> KVFGITGPVSTVGATAAENKLNDSLIQELKKEGSFETEQETANRVQVLKILQELAQRFVYEVSKKKNMSDGMARDAGGKIFTYGSYRLGVHGPGSDIDTLVVVPKHVTREDFFTVFDSLLRERKELDEIAPVPDAFVPIIKIKFSGISIALICARLDQPQVPLSLTLSDKNLLRNLDEKDLRALNGTRVTDEILELVPKPNVFRIALRAIKLWAQRRAVYANIFGFPGGVAWAMLVARICQLYPNACSAVILNRFFIILSEWNWPQPVILKPIEDGPLQVRVWNPKIYAQDRSHRMPVITPAYPSMCATHNITESTKKVILQEFVRGVQITNDIFSNKKSWANLFEKNDFFFRYKFYLEITAYTRGSDEQHLKWSGLVESKVRLLVMKLEVLAGIKIAHP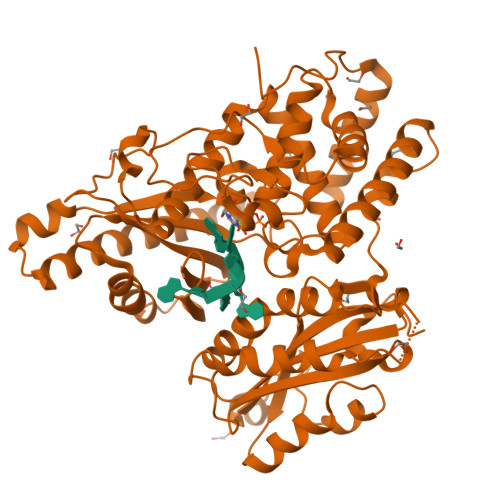FTKPFESSYCCPTEDDYEMIQDKYGSHKTETALNALKLVTDENKEEESIKDAPKAYLSTMYIGLDFNIENKKEKVDIHIPCTEFVNLCRSFNEDYGDHKVFNLALRFVKGYDLPDEVFDENEKRP In this work, we demonstrate the first ever high-resolution structure of co-assembly between a protein and buckminsterfullerene (C60), which suggests a simple structural mode for protein–fullerene co-organization. As in the protein-only structure, COP forms a canonical tetrameric anti-parallel coiled coil. Each tetramer presents four tyrosine residues (one per monomer) in exterior c positions of the coiled-coil heptad, and each of these engages a C60 moiety. One C60 is wedged between two Tyr residues donated by adjacent tetramers, such that two tetramers are needed to coordinate one C60.

Crystals from the resulting suspension grew within 24 h in several conditions, and three separate structures of the C60Sol–COP complex were resolved to 1.67, 1.76 and 2.35 Å, respectively. Furthermore, the three different COP–C60Sol co-crystals obtained under different conditions all produced effectively identical binding interfaces and assembly geometries, arguing that fullerene may have a strong preference for the observed coordination geometry. The interaction between COP and the fullerene group involves non-polar contacts, with C60 fitting perfectly into a symmetric hydrophobic cavity created by helices of two adjacent COP tetramers. The dominant contact appears to be the π–π aromatic stacking between C60 and Tyr9, donated by each tetramer, while several aliphatic carbons line the pocket to further support the bound pose. The water-solubilizing Tris-acid side chain of C60Sol is not visible in the electron density map. The group likely points into the solvated inner channel of the crystal and is highly mobile as the C60 core rapidly rotates around its centre. On the other hand, there is considerable difference in the arrangement of COP tetramers in the corresponding crystals: COP alone assembles into a body-centered cube, while C60Sol–COP has a honeycomb structure with parallel hexameric channels. In fact, in the fullerene bound structure, no contacts between adjacent COP tetramers occur outside of the C60-binding site. Inter-fullerene nearest-neighbour distances in the C60Sol–COP supercrystal alternate between 1.2 and 1.7 nm. On the other hand, C60Sol–COP supercrystals (of similar dimension as protein-alone crystals) exhibited high electrical conductance (1.40 × 10−7 S, corresponding to resistance of 7.14 × 106 Ω) with at least four orders of magnitude higher currents than in any of the controls.

>AEAESALEYAQQALEKAQLALQAARQALKA[2x]Cohesin is composed of two rod-shaped SMC proteins, Smc1 and Smc3, with a dimerisation interface at one end that is connected to an ABC-like ATPase domain via a 50-nm-long coiled coil. Interaction via their dimerisation domains produces a V-shaped Smc1/3 heterodimer whose two arms are connected by a central ‘hinge’ domain. The ATPase domains of all SMC proteins are separated from their hinge dimerisation domains by 50-nm-long coiled coils, which have been observed to zip up along their entire length and fold around an elbow, thereby greatly shortening the distance between hinges and ATPase heads. Cohesin’s association with DNA as well as its abilities to hold sisters together and extrude DNA loops are facilitated by three large hook-shaped HAWK (HEAT repeat proteins associated with kleisins) proteins; Scc2, Scc3, and Pds5.

The other is an aspartic acid on the surface of Smc1’s hinge domain that is replaced by an aromatic residue: smc1D588Y. Smc1D588 is located in the hinge domain, at the C-terminal end of a β strand that interacts in an antiparallel fashion with a strand in Smc3. Despite its proximity to the Smc1-Smc3 interface, D588 does not appear to contact Smc3 residues. To determine whether the smc1D588Y mutation alters the hinge structure, we introduced the equivalent mutation (D574Y) into an isolated mouse hinge. X-ray crystallography revealed that a clash between the tyrosine residue and neighbouring loop causes Y574 to instead swing out relative to the position of D574, causing a local conformational change of the mutated loop. Importantly, the change had little or no impact on the overall structure of the hinge. Y574 adopting the same conformation of D574 crashes with a neighbouring loop (right, D574Y). Tyr574 swings out relative to the position of D574 with a concomitant local conformational change of the mutated loop. Despite this, both D588Y and D588W reduced the amount of Smc1 hinge that co-precipitated with Smc3 hinges. To address whether Smc1D588Y affects dissociation of pre-assembled Smc1/3 hinge complexes, we co-expressed either WT Smc1 or Smc1D588Y hinge domains with Smc3 hinges, purified Smc1/3 complexes, and compared their persistence in the presence of a fivefold excess of SNAP-tagged Smc1 hinge domains. This revealed that the amount of Smc1D588Y associated with Smc3 hinges declined more rapidly in the presence of a WT competitor than WT Smc1, indicating that Smc1D588Y at least increases the off rate.

>[2x]DEINKELNQVMEQLGDARIDRQESSRQQRKAEIMESIKRLYPGSVYGRLIDLCQPTQKKYQIAVTKVLGKNMDAIIVDSEKTGRDCIQYIKEQRGEPETFLPLYYLEVKPTDEKLRELKGAKLVIDVIRYEPPHIKKALQYACGNALVCDNVEDARRIAFGGHQRHKTVALDGTLFQKSGVISGGASDLKAKARRWDEKAVDKLKEKKERLTEEL;>[2x]AAKREDLEKKQQLLRAATGKAILNGIDSINKVLEHFRRKGINQHVQNGYHGIVMNNFECEPAFYTCVEVTAGNRLFYHIVDSDEVSTKILMEFNKMNLPGEVTFLPLNKLDVRDTAYPETNDAIPMISKLRYNPRFDKAFKHVFGKTLICRSMEVSTQLARAFTMDCITLEGDQVSHRGALTGGYYDTRKSRLELQKDVRKAEEELGELEAKL> GSHMASRTPKKLSNIALTKETRQSSTDYNGFSRLAVDGNKNGDYGHHSVTHTKEDSPSWWEIDLAQTEELEKLIIYNRTDAE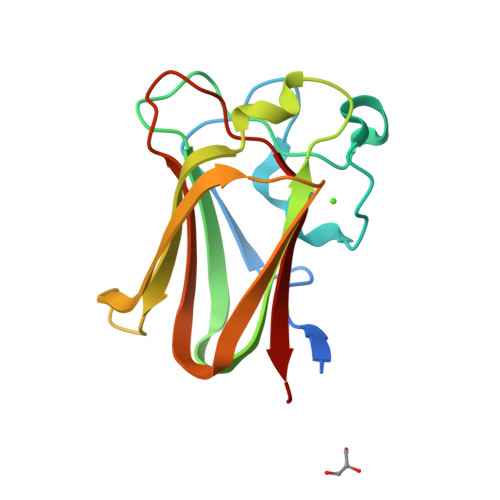IQRLSNFDIIIYDSNDYEVFTQHIDSLESNNLSIDLKGLKGKKVRISLRSAGIPLSLAEVEVYTYK> GSMADEATRRVVSEIPVLKTNAGPRDRELWVQRLKEEYQSLIRYVENNKNADNDWFRLESNKEGTRWFGKCWYIHDLLKYEFDIEFDIPITYPTTAPEIAVPELDGKTAMMYRGGKICLTDHFKPLWARNVPKFGLAHLMALGLGPWLAVEI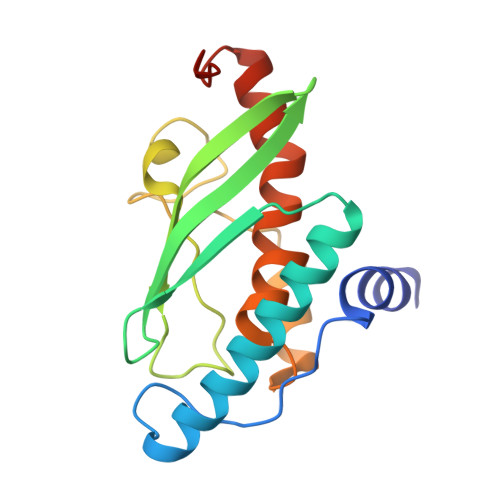PDLIQKGVIHHKEKCNQ> MKKVRLKELESRLQQVDGFEKPKLLL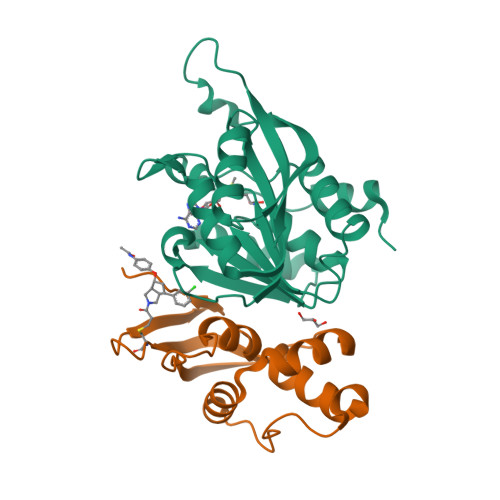EQYPTRPHIAACMLYTIHNTYDDIENKVVADLGCGCGVLSIGTAMLGAGLCVGFDIDEDALEIFNRNAEEFELTNIDMVQCDVCLLSNRMSKSFDTVIMNPPFGTKNNKGTDMAFLKTALEMARTAVYSLHKSSTREHVQKKAAEWKIKIDIIAELRYDLPASYKFHKKKSVDIEVDLIRFSF;> MKLLTHNLLSSHVRGVGSRGFPLRLQATEVRICPVEFNPNFVARMIPKVEWSAFLEAADNLRLIQVPKGPVEGYEENEEFLRTMHHLLLEVEVIEGTLQCPESGRMFPISRGIPNMLLSEEETES Phytochromes constitute a class of biological photoreceptors which harbor a linear methine‐bridged tetrapyrrole as a chromophore. The minimum functional entities are the photosensor (photosensory core module (PCM)) and an output module which is frequently a histidine kinase. In our previous studies, we intensively used the bathy phytochrome Agp2 from Agrobacterium fabrum as a model system, providing valuable insight into structure and reaction mechanism of phytochromes in general. Agp2 carries a biliverdin (BV) chromophore, which upon light excitation of the dark state Pfr photoisomerizes from ZZEssa to ZZZssa and subsequently runs via a sequence of thermal decays to Pr.

Additionally, we introduced a probe at Tyr205, a site that modulates the interactions between the B‐ and C‐ring propionic side chains during photoconversion—a critical step preceding propC deprotonation. For Y205oCNF, the crystal structure of Pfr was determined experimentally at a resolution of 1.79 Å. This structure reveals a very high overall agreement, even in the CBP, with a root‐mean‐square deviation (RMSD) of 0.28 Å compared to the WT Agp2 PCM. However, introducing the oCNF reporter group leads to an in‐place rotation of the Y205oCNF side chain by ≈20° compared to Tyr205 in WT‐Agp2 PCM. Together with the lack of the hydroxyl head group in oCNF, this alteration leads to a slight restructuring of the HB network around the BV chromophore in the Pfr crystal structure. On the one hand, a new water molecule is visible in the oCNF region of CBP, on the other hand, there is a slight shift in the head group of propC and a different rotamer orientation of Ser260. Since Tyr205 directly interacts with the propionic side chains, initially with propB and propC in Pfr and subsequently in Meta‐F solely with propB, one may readily rationalize the effects of the substitution on the chromophore, which is visible through small changes in the Y205oCNF Pfr crystal structure. One exception is Y205oCNF where the nitrile substituent in ortho position in Y205oCNF cannot replace the hydroxyl group of Tyr and its HB interactions, first with propB and propC (Pfr) and later solely with propB (Meta‐F). In Y205oCNF, this coupled process is not completed at pH 7.8. It requires an increase of the pH to 9.0 to achieve the same signal pattern as in the other variants and in WT Agp2‐PCM.

>[2x]MASTDYHVDLTNCDREPIHIPGYIQPHGCLIACDNAMRMVLRHSENCGELLGLEGDLNGRTAEDVLGKKLVHDLRNALTVTGRTTRPAMLPAMETSDGRSFDISLHRYKSTTIIEFEPSGSDAQPLGTARKMVDRIREADSVESLISRTTRLVKATLGYDRVMIYRFQEDGAGKVVSEAKQPELESFLGQYFPASDIPQQARALXLKNTLRIISDASGTRIPVLPAVDVSGEPLDLSYAHLRSVSPIHCEYLRNMGVAASMSISVIVDGALWGLIACHHYSPRVLSMPVRIAAEMFGEFFSMHLQVLKQKRRLDTINHAHAALDRFLRLAAHHANIEELLVDSFQDFADLMPCDGVGLWVGNNWHGHGATPPHDAIPRLARFVASASEGRVWATHALSQAIPEAEIYAGTAAGMLAIPLSQVKSDYLLFFRKEIVQNLNWAGNPEKSYETGPMGDRLTPRKSFAIWKETVRLQAQPWSEADREIAEAARIALVEVAFHHSEHHHHHH>GMIRVMATGVFDILHLGHIHYLKESKKLGDELVVVVARDSTARNNGKIPIFDENSRLALISELKVVDRAILGHEGDMMKTVIEVKPDIITLGYDQKFDEAELQSKINKLGITVKIVRISKYDGQLNSSSSVRKKI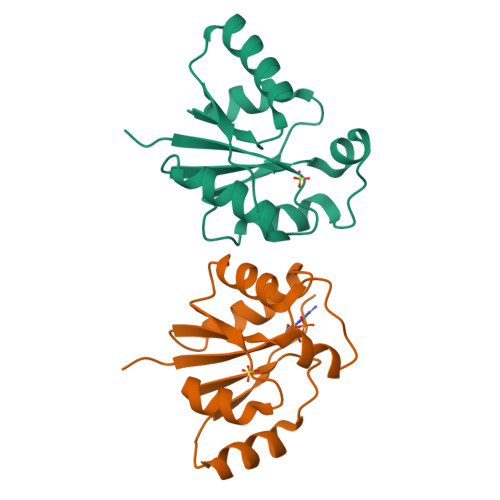MELIGERY[2x]>MGLSLPKEKGLILCLWSKFCRWFQRRESWAQSRDEQNLLQQKRIWESPLLLAAKDNDVQALNKLLKYEDCKVHQRGAMGETALHIAALYDNLEAAMVLMEAAPELVFEPMTSELYEGQTALHIAVVNQNMNLVRALLARRASVSARATGTAFRRSPCNLIYFGEHPLSFAACVNSEEIVRLLIEHGADIRAQDSLGNTVLHILILQPNKTFACQMYNLLLSYDRHGDHLQPLDLVPNHQGLTPFKLAGVEGNTVMFQHLMQKRKHTQWTYGPLTSTLYDLTEIDSSGDEQSLLELIITTKKREARQILDQTPVKELVSLKWKRYGRPYFCMLGAIYLLYIICFTMCCIYRPLKPRTNNRTSPRDNTLLQQKLLQEAYMTPKDDIRLVGELVTVIGAIIILLVEVPDIFRMGVTRFFGQTILGGPFHVLIITYAFMVLVTMVMRLISASGEVVPMSFALVLGWCNVMYFARGFQMLGPFTIMIQKMIFGDLMRFCWLMAVVILGFASAFYIIFQTEDPEELGHFYDYPMALFSTFELFLTIIDGPANYNVDLPFMYSITYAAFAIIATLLMLNLLIAMMGDTHWRVAHERDELWRAQIVATTVMLERKLPRCLWPRSGICGREYGLGDRWFLRVEDRQDLNRQRIQRYAQAFHTRGSEDLDKDSVEKLELGCPFSPHLSLPMPSVSRSTSRSSANWERLRQGTLRRDLRGIINRGLEDGESWEYQI[4x]

TRPV6 is a representative of the vanilloid subfamily of transient receptor potential (TRP) channels that serves as an entry gate for capturing dietary calcium ions in the gut1–3. In a nutshell, hTRPV6 is assembled of four subunits and contains a transmembrane domain (TMD) with a central ion channel pore and an intracellular skirt that is mostly built of ankyrin repeat domains connected by the three-stranded β-sheets, N-terminal helices, and C-terminal hooks. The TMD is composed of six transmembrane helices S1–S6 and a re-entrant pore loop (P-loop) between S5 and S6. As in all representatives of the tetrameric ion channel family, the ion-conducting pore of TRPV6 has two narrow regions, the selectivity filter formed by the extended regions of the P-loop and the gate formed by the S6 bundle crossing, separated by the central cavity in the middle.

The first, smaller population of particles yielded a 2.71-Å cryo-EM map that showed four-fold rotational symmetry (C4) and represented a typical genistein-free apo state, hTRPV6Open. For the 4-fold symmetrical hTRPV6Open homotetramer, we built a molecular model of a single subunit, including residues 28–637 and excluding residues 1–27 (N-terminus) and 638–725 (C-terminus), which were not clearly resolved in the cryo-EM map. In hTRPV6Open, the pore is wide open and its narrow region is lined by residues N572 and I575. This conformation is the same as in the previously published open-state structures of TRPV6, independent of whether they had C-terminus truncated or not and whether the protein was purified in different types of detergents, nanodiscs or amphipols, strongly supporting our initial assignment of hTRPV6Open to the open conducting state. In the open state, S6 undergoes an α-to-π transition, which produces a π-bulge in the middle of this helix. Formation of the π-bulge is accompanied by a ~100° rotation of the C-terminal portion of S6, which brings a completely different set of residues to face the pore and opens it for ion conduction. When binding to the open TRPV6 channel perpendicularly to the central pore axis, genistein molecules pull one diagonal pair of subunits (A/C) asymmetrically towards the channel center. This motion breaks the interactions between D489 in S5 and T581 in S6 as well as Q473 in the S4–S5 linker and R589 in the TRP helix, which stabilize the energetically unfavorable α-to-π transition in S6 and the open-pore conformation, respectively. TRPV6 is a constitutively open ion channel.N-(4-{[(2,4-diaminopteridin-6-yl)methyl](hydroxymethyl)amino}benzene-1-carbonyl)-L-glutamic acid | C20 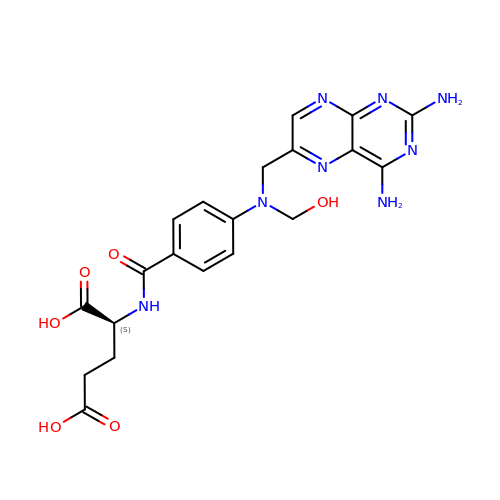H22 N8 O6 | KWWKVKGHDTULAH-ZDUSSCGKSA-N> IP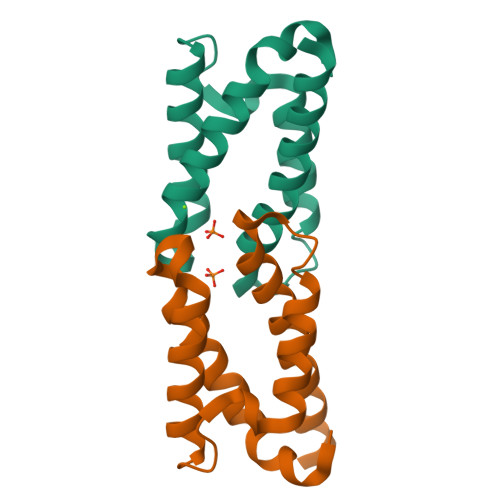AGELQIIDKIDAAFKVAATAAATAPADDKFTVFEAAFNKAIKETTGGAYDTYKCIPSLEAAVKQAYAATVAAAPQVKYAVFEAALTKAITAMSEVQKVSQ> ALVIAFIGKNGAVMAGDMREITFEGEKPDREKLEKELYSGSIVTDEEMQKKAEEFGVKITVADCKEKVSERNGVLVGEVSSAEGGVVKKRRLYASAGNFAIAELINTEMTLTSQGKGSNFIAFGNEFTKQVANKCFKDNWTKKSNLQDAVKILILCMETVARKTASVSKQFMIVQTASNADVLKVVEKDRNS;> RELASKDPGAVDAKPLVVEI

The discovery of peptide ligase activity in the Connectase family of enzymes (CETs) from archaea has expanded protease repurposing strategies. However, original CETs exhibit significant residual protease activity, leading to nonprocessive (reversible) ligation and limiting their application. In this study, we present crystal structures of a highly active protein ligase from Methanococcus maripaludis (MmCET) in both its apo- and substrate-bound forms. By determining the crystal structure of MmCET, both with and without a preferred peptide substrate at its catalytic transition state, we uncovered the essential elements responsible for the high-precision substrate recognition of N-terminal motifs.

Swapping two amino acids at the P4’ and P7’ positions (F → V, and D → K, respectively) of MmCET (bold) significantly enhanced the ligation efficacy (peptide sequence: RELASKD|PGAVDAKPLVVEI). The resulting structure at ∼2.1 Å resolution revealed the atomic details of how MmCET formed intricate interactions with its preferred substrates. Given the overall elongated shape, its recognition by MmCET can be likened to the jaw of a crocodile biting a buffalo leg. Notably, the C-terminal substrate pocket of MmCET exhibits relatively loose interactions with the bound peptide. In contrast, the N-terminal substrate recognition groove features opposite side chains that form specific interactions with the substrate. Side chains from residues 88–103, as well as N119, I121, and H123, form the upper surface of this groove, while side chains from α-helix 3 (residues 125–140) constitute the bottom surface. The bound peptide substrate within this N-terminal binding groove adopts a β-sheet secondary structure, interacting with these upper and lower surface side chains. Overall, the N-terminal substrate recognition groove (reading the P4′–P13’ residues from the substrate) forms a set of highly specific interactions, resembling the shapes of “teeth” inside the crocodile jaw, that only permitted binding of substrates with a well-defined combination of amino acids. The peptide bond after the aspartic acid residue at the P1 position could be attacked by threonine 1 from MmCET (note that the T1A in the actual crystal structure renders the enzyme inactive), forming a transition state complex in which the C-terminal substrate is directly linked to Thr1 of MmCET via a peptidyl bond, while proline at the P1’ position is cleaved. Indeed, by observing the conformation of a peptide substrate captured in our complex structure, we noticed that the Pro-Gly-Ala sequence at the P1′–P3′ positions is highly unstable (orange color) based on its bond angle constraints.4-[3-(1,4-diazepan-1-ylcarbonyl)-4-fluorobenzyl]phthalazin-1(2H)-one | C21 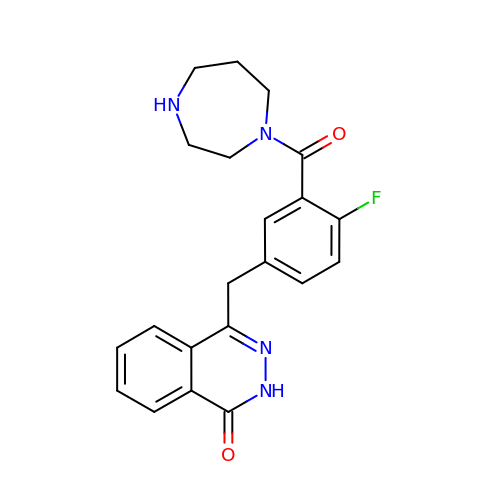H21 F N4 O2 | HGEPGGJUGUMFHT-UHFFFAOYSA-N OCTYL-PHOSPHINIC ACID 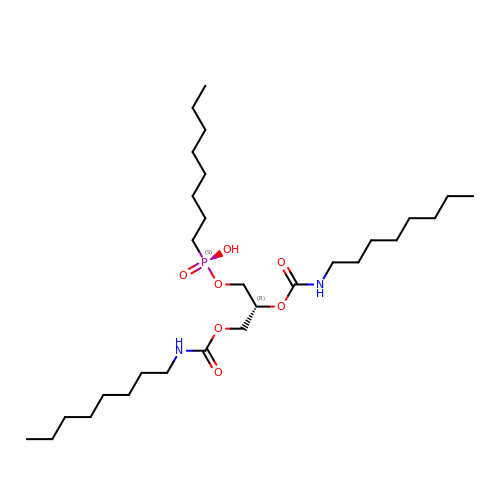1,2-BIS-OCTYLCARBAMOYLOXY-ETHYL ESTER | C29 H59 N2 O7 P | QRWKUAOYWKHOGP-HHHXNRCGSA-N> MTSYTYQATPMDGTLKTMLERWAADSNMQLSYNLPSDYTLIGPVSAISTTSVQQAATELSAV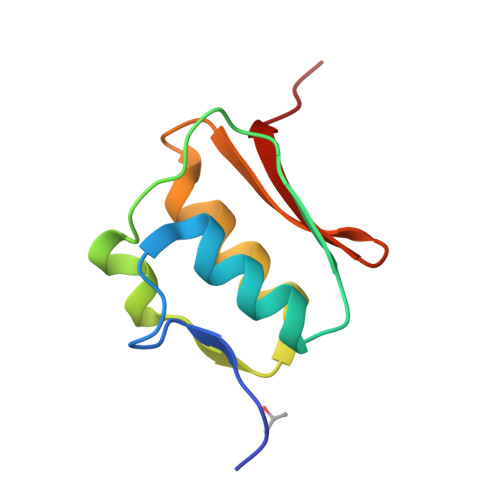YAAQGVSVSVSANKLLVQPVPVS> MSGDSVAPHQRAACEQLHSEYKQCLAKNGRTHFSACTDFHSKLRACENMLGTSYCIDEGINLMKCTKNPDPSFCAKEFV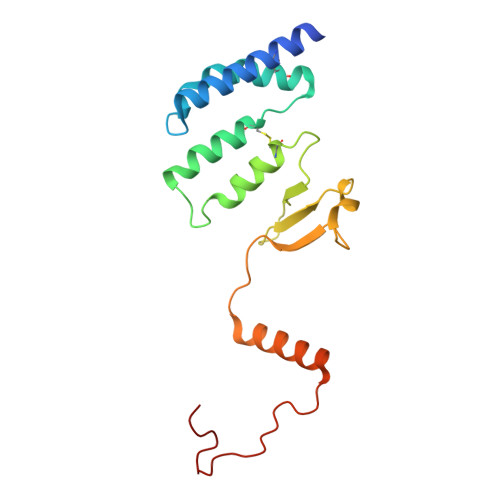AMRECNRPQGPHLVLSSSPSSPPHYELRPEVKHLYNVDSTDLGSAVAPVRSKEQLDRVADSLKADLNLPGYGHIPYKWESLRPNPGA CYCLOHEXANE PROPIONIC ACID | C9 H16 O2 | 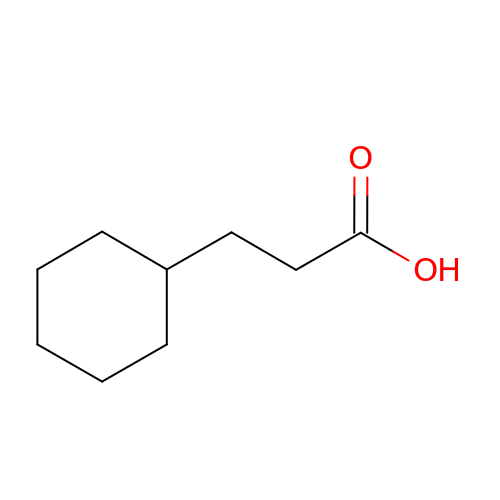HJZLEGIHUQOJBA-UHFFFAOYSA-N> XG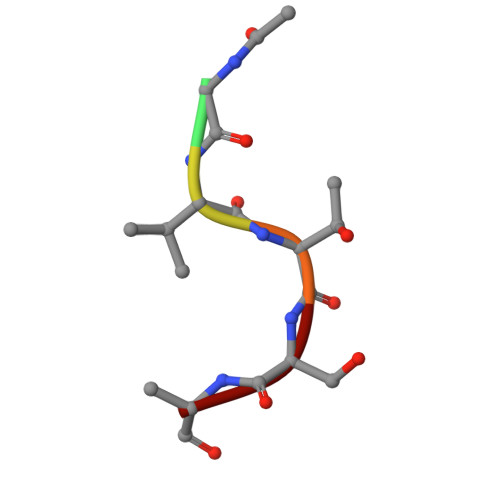VTSA>[2x]METFGEKTTSTAPPVAELHLHIEGTLQPELIFALAERNGIELPYEDIEELREKYEFTDLQSFLDLYYANMAVLQTEQDFTDMTRAYLERAAAGGVRHAEIMMDPQAHTSRGVALETCVNGVANALATSEEDFGVSTLLIAAFLRDMSEDSALEVLDQLLAMH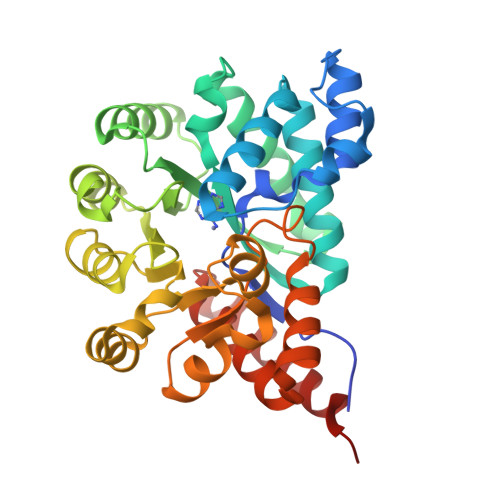APIAGIGLDSAEVGNPPSKFERLYQRAAEAGLRRIAHAGEEGPASYITEALDVLHVERIDHGIRCMEDTDVVQRLVAEQVPLTVCPLSNVRLRAVDKLADHPLPEMLAIGLNVCVNSDDPAYFGGYVDDNFEQLVKVLEFSVPEQATLAANSIRSSFASDARKAVLLDEVTEWVKASVTPA>[6x]GSAPVTVTRFVDASPTGYDWRADWVKGFPIDSSCNATQYNQLSTGLQEAQLLAEHARDHTLRFGSKSPFFRKYFGNETASAEVVGHFDNVVGADKSSILFLCDDLDDKCKNDGWAGYWRGSNHSDQTIICDLSFVTRRYLTQLCSSGYTVSKSKTNIFWAGD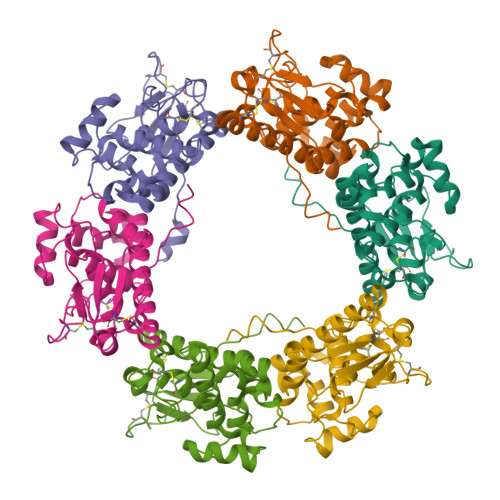LLHRFWHLKSIGQLVIEHYADTYEEVLELAQENSTYAVRNSNSLIYYALDVYAYDVTIPGEGCNGDGTSYKKSDFSSFEDSDSGSDSGASSTASSSHQHTDSNPSATTDANSHCHTHADGEVHC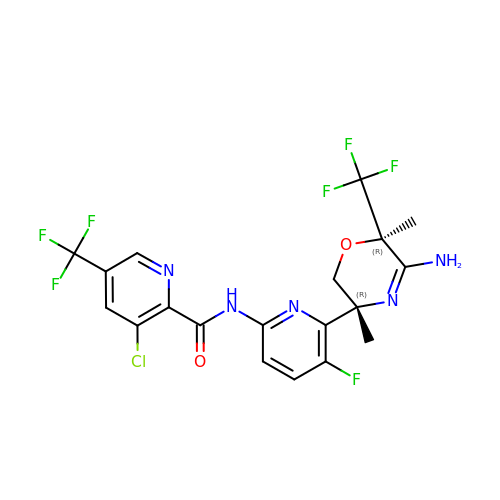~{N}-[6-[(3~{R},6~{R})-5-azanyl-3,6-dimethyl-6-(trifluoromethyl)-2~{H}-1,4-oxazin-3-yl]-5-fluoranyl-pyridin-2-yl]-3-chloranyl-5-(trifluoromethyl)pyridine-2-carboxamide | C19 H15 Cl F7 N5 O2 | PSBBWFNMHDUTRH-DLBZAZTESA-N> GSHMELTPDQQTLLHFIM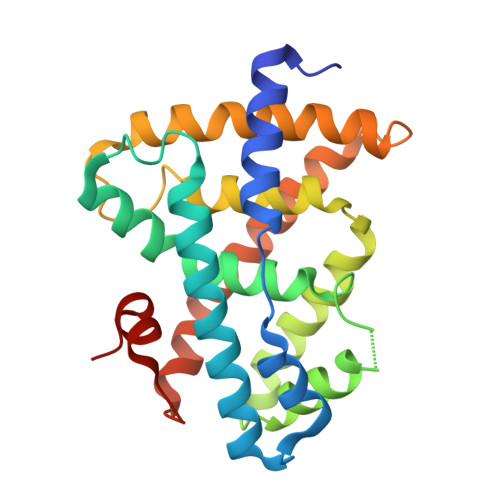DSYNKQRMPQEITNKILKEEFSAEENFLILTEMATNHVQVLVEFTKKLPGFQTLDHEDQIALLKGSAVEAMFLRSAEIFNKKLPSGHSDLLEERIRNSGISDEYITPMFSFYKSIGELKMTQEEYALLTAIVILSPDRQYIKDREAVEKLQEPLLDVLQKLCKIHQPENPQHFACLLGRLTELRTFNHHHAEMLMSWRVNDHKFTPLLCEIWDVQ4,5-bis(chloranyl)-3-nitro-1~{H}-pyridazin-6-one 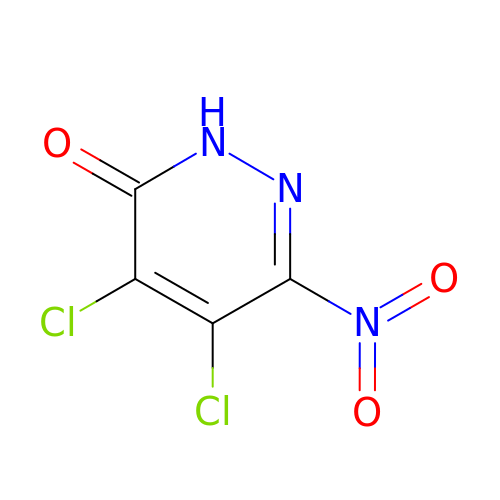| C4 H Cl2 N3 O3 | SCNATHDZNWMBOX-UHFFFAOYSA-N> GAAAAMSICPHIQQVFQNEKSKDGVLKTCNAARYILNHSVPKEKFLNTMKCGTCHEINSGATFMCLQCGFCGCWNHSHFLSHSKQIGHIFGINSNNGLLFCFKCEDYIGNIDLINDAILAKYWDDVCTKTMVPSMERRDGLSGLINMG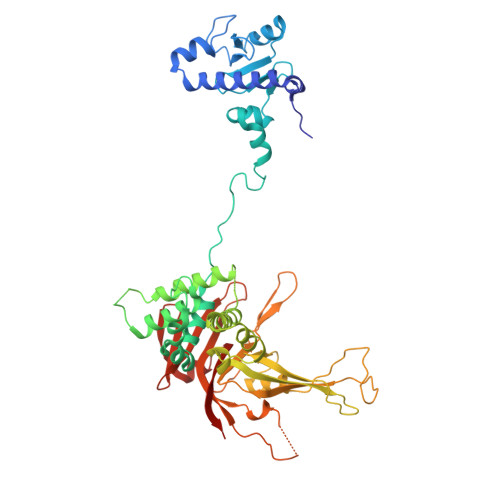NTCFMSSILQCLIHNPYFIRHSMSQIHSNNCKVRSPDKCFSCALDKIVHELYGALNTKQASSSSTSTNRQTGFIYLLTCAWKINQNLAGYSQQDAHEFWQFIINQIHQSYVLDLPNAKEVSRANNKQCECIVHTVFEGSLESSIVCPGCQNNSKTTIDPFLDLSLDIKDKKKLYECLDSFHKKEQLKDFNYHCGECNSTQDAIKQLGIHKLPSVLVLQLKRFEHLLNGSNRKLDDFIEFPTYLNMKNYCSTKEKDKHSENGKVPDIIYELIGIVSHKGTVNEGHYIAFCKISGGQWFKFNDSMVSSISQEEVLKEQAYLLFYTIRQVN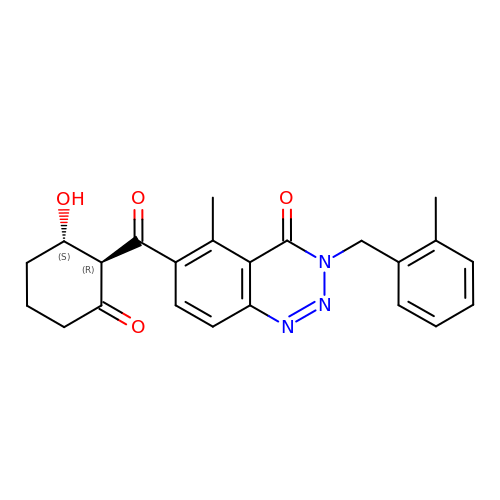5-methyl-3-[(2-methylphenyl)methyl]-6-[(1~{R},2~{S})-2-oxidanyl-6-oxidanylidene-cyclohexyl]carbonyl-1,2,3-benzotriazin-4-one | C23 H23 N3 O4 | WGYHEGBXADFJIU-GHTZIAJQSA-N>[2x]GAKQGEVSKAASADSTTEGTPADGFTVLSTKSLFLGQKLNLIHSEISNLAGFEVEAIINPTNADIDLKDDLG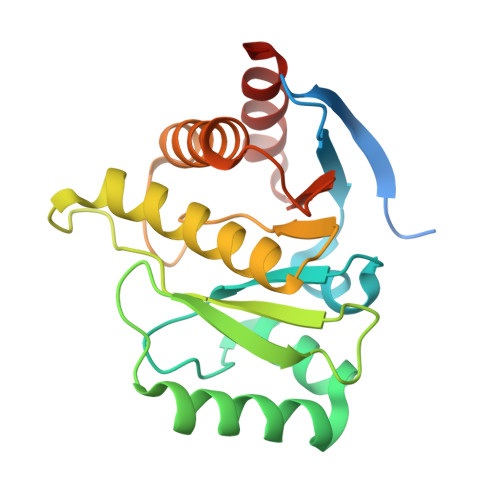NTLEKKGGKEFVEAVLELRKKNGPLEVAGAAVSAGHGLPAKFVIHCNSPVWGADKCEELLEKTVKNCLALADDKKLKSIAFPSIGSGRNGFPKQTAAQLILKAISSYFVSTMSSSIKTVYFVLFDSESIGIYVQEMAKLDAN N-(3,3-DIPHENYLPROPYL)PYRROLIDINE-1-CARBOXAMIDE 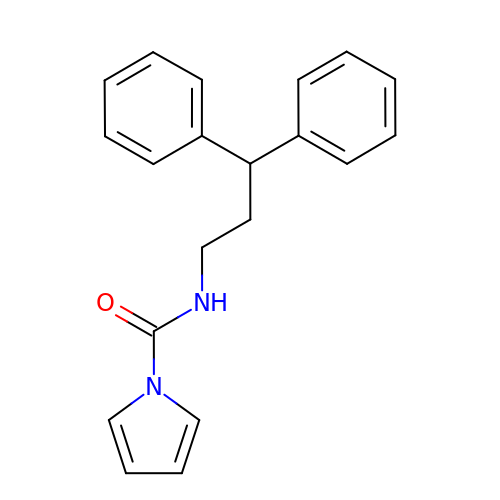| C20 H20 N2 O | HEHFNRQOOMVVBY-UHFFFAOYSA-N3-(2-hydroxyphenyl)benzoic acid | C13 H10 O3 | 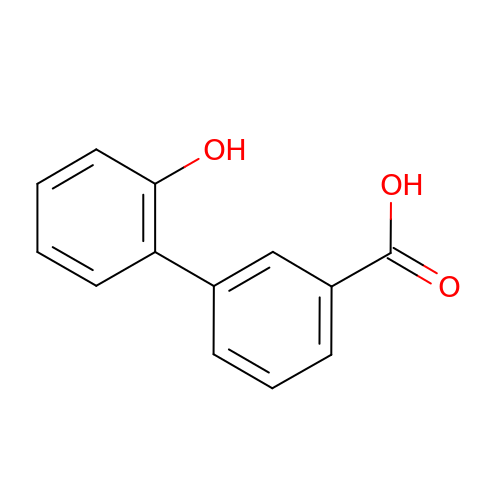OCZVWZVTEQXRPI-UHFFFAOYSA-N>[2x]MKESRAKKFQRQHMDSDSSPSSSSTYCNQMMLLRNMTQGRCKPVNTFVHEPLVDVQNVCFQEKVTCKNGQGNCYKSNSSMHITDCRLTNGSRYPNCAYRTSPKERHIIVACEGSPYVPVHF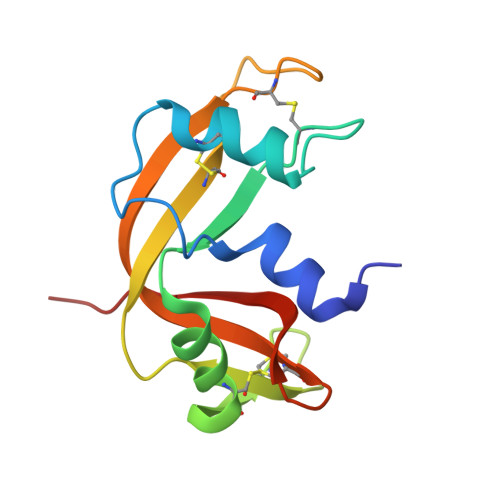DASVEDST> MASMTGGQQMGRGSMSRDPLPFFPPLYLGGPEITTENCEREPIHIPGSIQPHGALLTADGHSGEVLQMSLNAATFLGQEPTVLRGQTLAALLPEQWPALQAALPPGCPDALQYRATLDWPAAGHLSLTVHRVGELLILEFEPTEAWDSTGPHALRNAMFALESAPNLRALAEVATQTVRELTGFDRVMLYKFAPDATGEVIAEARREGLHAFLGHRFPASDI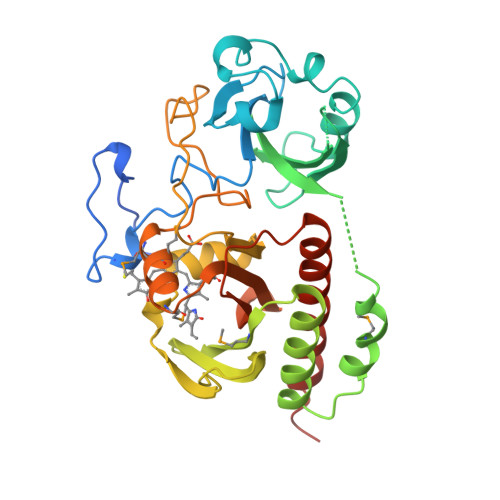PAQARALYTRHLLRLTADTRAAAVPLDPVLNTQTNAPTPLGGAVLRATSPMHMQYLRNMGVGSSLSVSVVVGGQLWGLIACHHQTPYVLPPDLRTTLEYLGRLLSLQVQVKEAHHHHHH> MFRNILSLVTKPSKLSQKTFYNFAAAKNEVQVSKKQQQAGAKRDLTQYVEGQIVNRNQLTLKKQEDIEQYVLKLVRGYFRTTNKQGLNINSVLQDHGLDEFDSIELAMQ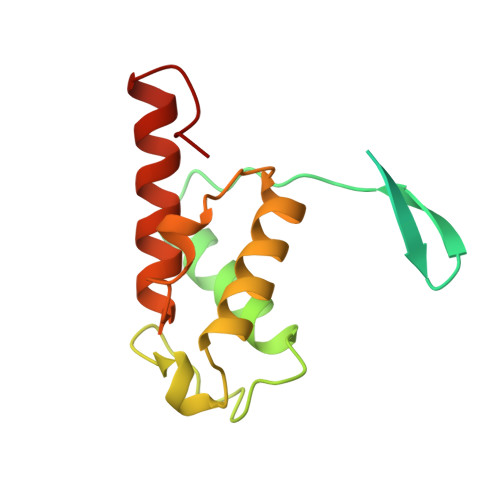VEEDLGYVISAETIPVLNKVKHFVNYINHVEQFKAENGKAPIA> 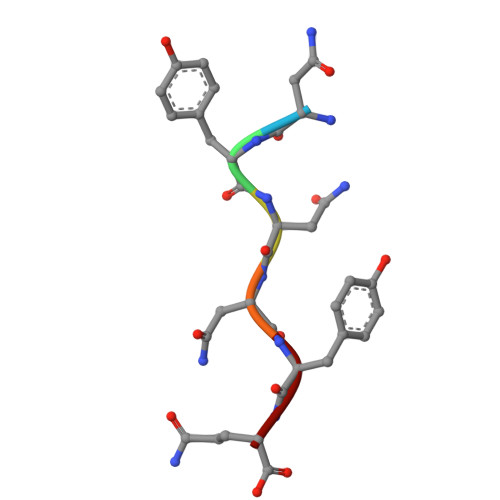NYNNYQ ALG-2 (apoptosis-linked gene 2) is a 22-kDa protein of 191 amino acid residues containing five serially repetitive EF-hand-type helix-loop-helix Ca2+-binding motifs (EF1 to EF5) and it belongs to the penta-EF-hand (PEF) family, including the calpain small subunit, sorcin, grancalcin and peflin in mammals. ALG-2 (a gene product of PDCD6) belongs to the penta-EF-hand (PEF) protein family and Ca2+-dependently interacts with various intracellular proteins including mammalian Alix, an adaptor protein in the ESCRT system. X-ray crystal structures of various PEF proteins including ALG-2 have common features: the presence of eight α-helices and dimer formation via paired EF5s that are positioned in anti-parallel orientation. Binding of Ca2+ (or Zn2+) to EF3 enables the side chain of R125, present in the loop connecting EF3 and EF4, to move enough to make a primary hydrophobic pocket (Pocket 1) accessible to the critical PPYP motif found in Alix.

An alternatively spliced shorter isoform, designated ALG-2ΔGF122, lacks Gly121Phe122 and does not bind Alix, but the structural basis of the incompetence has remained to be elucidated. An asymmetric unit of the crystal of des3-23ALG-2ΔGF122 in the Ca2+-bound form contained two ALG-2 molecules (A and B) as a dimer. In des3-23ALG-2ΔGF122, however, the deletion of Gly121Phe122 caused loss of the third turn in α5 that corresponds to the exiting helix of EF3 (magenta). In the structure of des3-23ALG-2ΔGF122 in the Ca2+-bound form, however, NH2R123 (corresponding to NH2R125 in wild-type ALG-2) did not form such a hydrogen bond. The side chain extended outwardly from the loop as in the case of the structure of the metal-free form, but the spatial positions of the side chains between R123 and Y122 were closer in the equivalent residues in the metal-free ALG-2 (R125 and Y124). Three calcium ions were found in EF1, EF3 and EF5 of des3-23ALG-2ΔGF122 at the canonical EF-hand coordination positions (x, y, z, -y, -x and -z), though water molecules at the -x positions in EF1 and EF3 were absent and no amino acid residue coordinated at the -z position in EF5. On the other hand, the side chain directed toward Pocket 1 in Ca2+-bound des3-23ALG-2ΔGF122, but it did not fully block the entry path of Pocket 1 as in the case of metal-free ALG-2. Since S120 is located within α5 in ALG-2 but is placed at the end of the truncated helix in ALG-2ΔGF122, an α-helix-supporting hydrogen bond between OS120 and NG121 (G123 in wild type) is disrupted. This causes a change in the spatial orientation of OS120, and the hydrogen bond with NH2R125 in wild-type ALG-2 is lost in NH2R123 in ALG-2ΔGF122. The distance between the Cα atoms of Y122 and T160 (facing Pocket 1) is shorter in the crystal structure of des3-23ALG-2ΔGF122 (8.7 Å) than that between the corresponding Y124 and T162 in the Ca2+-bound (9.9 Å) and metal-free structure of des3-20ALG-2 (9.0 Å), indicating a narrower Pocket 1 in the isoform.

>ADQSFLWNVFQRVDKDRSGVISDTELQQALSNGTWTPFNPVTVRSIISMFDRENKAGVNFSEFTGVWKYITDWQNVFRTYDRDNSGMIDKNELKQALSGYRLSDQFHDILIRKFDRQGRGQIAFDDFIQGCIVLQRLTDIFRRYDTDQDGWIQVSYEQYLSMVFSIV[2x]> MAKVLCVLYDDPTSGYPPLYARNAIPKIERYPDGQTVPNPKHIDFVPGELLGCVSGELGLRSYLEDLGHTFIVTSDKEGPNSVFEKELPDADIVISQPFWPAYLTAERIAKAKKLKLALTAGIGSDHVDLNAAIKAGITVAEETFSNGICVAEHAVMMILALVRNYLPSH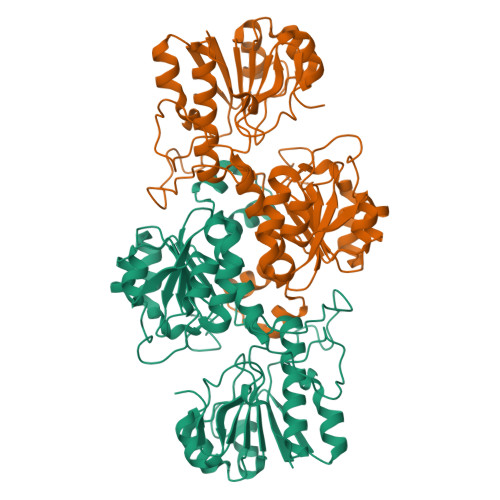KIAEEGGWNIADCVSRSYDLEGMHVGTVAAGRIGLAVLRRLKPFDVKLHYTARHRSPRAIEDELGLTYHATAEEMAEVCDVISIHAPLYPATEHLFNAKVLNKMRHGSYLVNTARAEICDRDDIVRALESGQLAGYAGDVWFPQPAPANHPWRNMPHNGMTPHMSGSSLSGQARYAAGTREILECWFENRPIRDEYLIVSNGKLAGTGAKSYGVGEAPKGK benzo[b][1]benzazepine-11-carboxamide | C15 H12 N2 O | 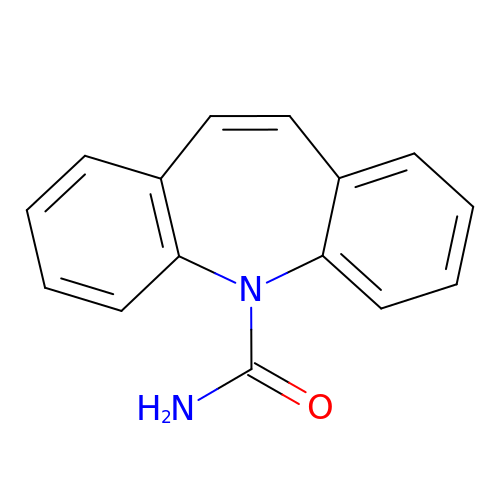FFGPTBGBLSHEPO-UHFFFAOYSA-N> HHHHHH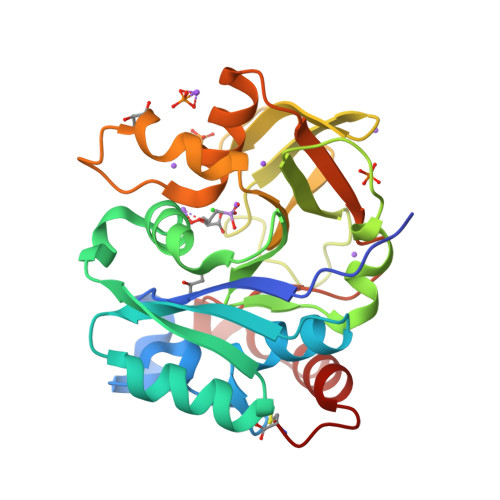FQGAMREAIVLASGAGKRLRSVTGDVPKVFYRFDGCELVKYPMISLMKNGVERFVLVVSEGYRDLGEKVLNDLGVEGIVVENKKVELGNAYSFFLSEPYVESEKFFLSCGDSLFPPSALKSAFSEDEFHIKLGVSKRSDLIDPEKASKVLVNENRIVKIGKRIDQYNYFDTGVFVMTKKVYSLKESFSWTEDISLYHVLQKAVDTGMIVKVFDFGNALWTEIDSPADLNSKVYELMSKIKEGVAC>PLRMGGNGQLQYWPFSSSDLYNWKNNNPSFSEDPGKLTALIESVLTTHQPTWDDCQQLLGTLLTGEEKQRVLLEARKAVRGNDGRPTQLPNEVDAAFPLERPDWDYTTQRGRNHLVLYRQLLLAGMQNAGRSPTNLAKVKGITQGPNESPSAFLERLKEAYRRYTPYDPEDPGQETNVSMSFIWQ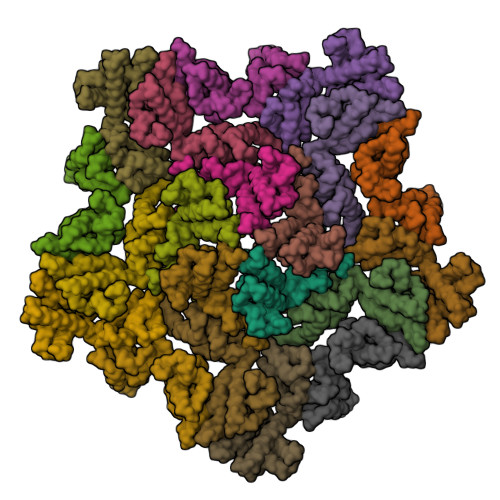SAPDIGRKLERLEDLKSKTLGDLVREAEKIFNKRETPEEREERIRRETEEK[4x]(3R)-3-[(1R)-1-azanylethyl]nonanedioic 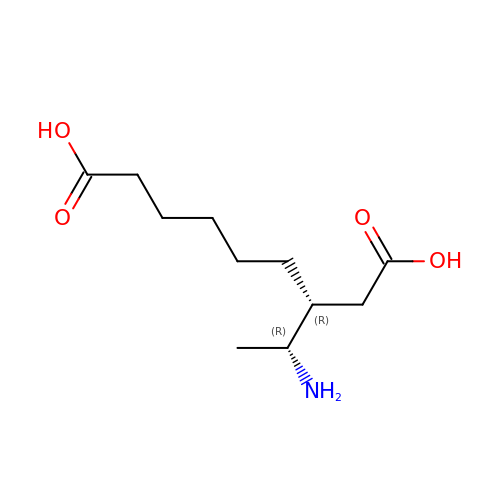acid | C11 H21 N O4 | NHQUUILSXUJSSP-RKDXNWHRSA-N> THVDLGLASANVDFAFSLYKQLVLKAPDKNVIFSPLSISTALAFLSLGAHNTTLTEILKGLKFNLTETSEAEIHQSFQHLLRTLNQSSDELQLSMGNAMFVKEQLS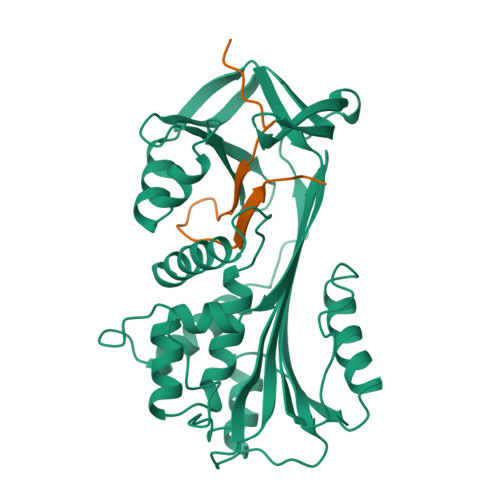LLDRFTEDAKRLYGSEAFATDFQDSAAAKKLINDYVKNGTRGKITDLIKDLDSQTMMVLVNYIFFKAKWEMPFDPQDTHQSRFYLSKKKWVMVPMMSLHHLTIPYFRDEELSCTVVELKYTGNASALFILPDQDKMEEVEAMLLPETLKRWRDSLEFREIGELYLPKFSISRDYNLNDILLQLGIEEAFTSKADLSGITGARNLAVSQVVHKAVLDVFEEGTERSAATAVKITLL;> VETRTIVRFNRPFLMIIVPTDTQNIFFMSKVTNPKQA>[2x]VSPNYDKWEMERTDITMKHKLGGGQYGEVYEGVWKKYSLTVAVKTLKEDTMEVEEFLKEAAVMKEIKHPNLVQLLGVCTREPPFYIITEFMTYGNLLDYLRECNRQEVNA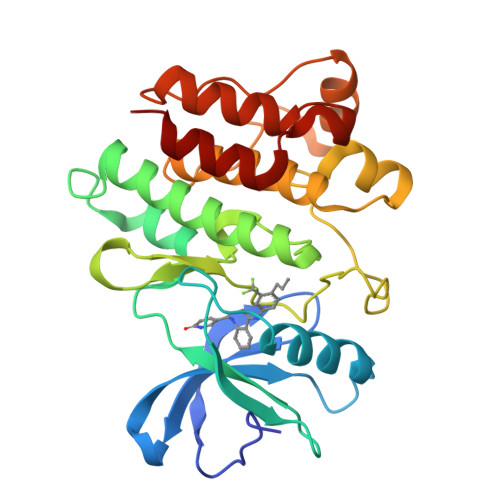VVLLYMATQISSAMEYLEKKNFIHRDLAARNCLVGENHLVKVADFGLSRLMTGDTYTAHAGAKFPIKWTAPESLAYNKFSIKSDVWAFGVLLWEIATYGMSPYPGIDLSQVYELLEKDYRMERPEGCPEKVYELMRACWQWNPSDRPSFAEIHQAFETMF> AVTCGQVDANLAPCVPFLTQGGEPGAACCSGVKTLNGNAQSPDDRKTACNCIKA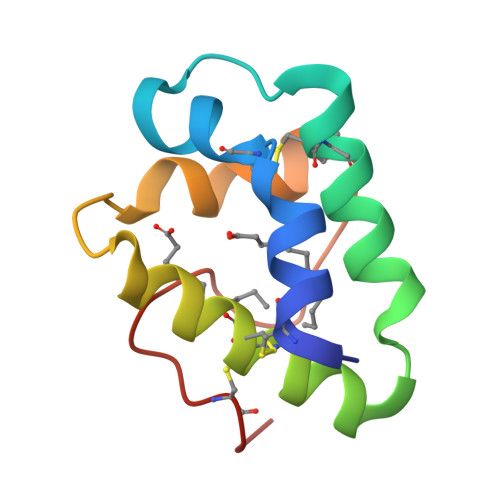AANRYPNLKDDAAQSLPSKCGISLNVPISRTINCDTIS>MASTIASEDARYRQSSQYELWSFSPSQLASMREKTNAAARARITERLLSMPNPSNTASAPTSSANTPDPDGVSTPTLPEFLTPAEELLLVTFYTAELLRAGDHADMSDEIKATAATFFKRFYITNSIMTYPPQEMLLVALFFGCKAEGAFPSISDFAKTFGRERPEEILAGEFLLCQGIRFALDVKHPFRALRGAIMELSTLPDVEPARLVAAEQRAREILRFSPLITDAYFHFTPSQIMLAALSLADRGLAERLIQDTFHYVAPQPSSGTDTPATSGVETPSGASASISLHKRTASPSSGSLEDKAAVIGSHVRDKVLGTIEACRDMLSKELPERREHWNNKTVYKAQIQPIRKKLNKCRDPDRWNLVELQRIRREQASRKGFDSDDEGEGRTKGGSLEDDAAVFGVPKKKKQLEDPFGPPLAG[2x];>MAASPLIAPPTDALQQSRPGSTSSPFKRQPQQPSQPPSSTAPSSSNANDTPQLGSRPPNITIANVTSAPFSSRPAITPDPVEQMNEAEKRKYIKGKKLGEGTYANVYLGHSRDDPNFKVAIKKIKVQAQYKDGMAPDAVRELKYLRELRGHPNIIGLISVFSSKDQNLNLVLEYLPLGD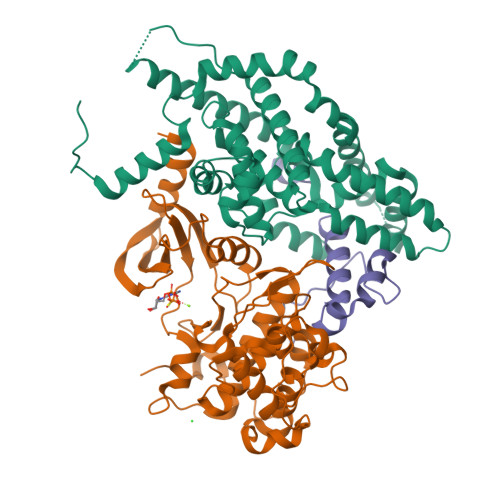LEMLIRDVERVRYGAADIKAWMGMLTRAVWWCHENFILHRDIKPNNLLIAADGEVKLADFGLARSFADPGRRMTANVITRWYRPPELLFGARHYGGAVDIWSVGMVFAELIIRSPFLPGNTEMEQITLICKHIGTPTEENWPGVSKLPEWWDPMEEPIPVWGKDAYMARFGAVGSEGVDLLWRTLQLDPKKRITAREMLEHRWWRTDPKPTRKEDLPKKSGGEDKMGADLKRRPGMVEDENGPRGSKVARKLDFGQLK[2x];>[2x]GPYDPFGGMEFVPSRYRVREELNHPSLDKYRIDQQHITGGYSFLDYISRAMFEAFAGLAVFIEDEKEAG(2S,6S,11S)-6,11-dimethyl-3-(3-methylbut-2-en-1-yl)-1,2,3,4,5,6-hexahydro-2,6-methano-3-benzazocin-8-ol | C19 H27 N O | 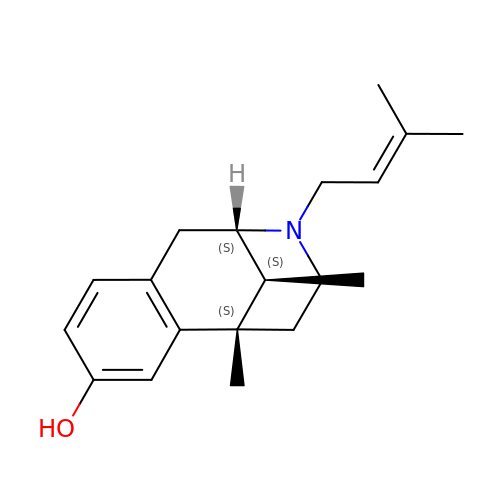VOKSWYLNZZRQPF-CCKFTAQKSA-N> MEEILDRIINPLSAKPLTKKEHIYTSLVLQSSQSLILSACPSLQSQRQFCSFEYHQQFIDWCFFNKKRTDWCLALSFYQYLSYKNEQVSVEILKELIHLACSQWTYAD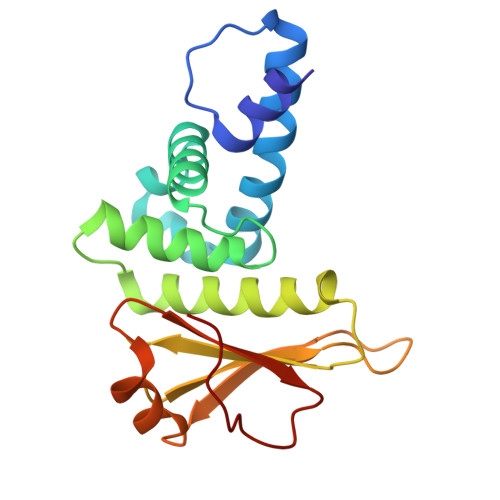KSTNQTVVICHTRLPSMVFGGNKSLFAQEFREVFLLETEQLKPFIQSHVPDGYFVYWILRDDSEYPSTMGEK> SNMYGFGTAATGEGSGVLFGNPHWYWKGPDRFYQAQLTIDGEANVSGVSFL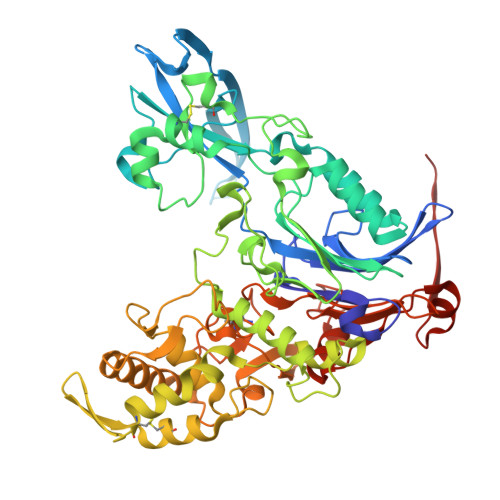GLPVIQIGFNDSVAWSHTVSTARRFGFFQLSLVQGEPTSYLRDGVPVKMKPATITVPSRNADGSVSDVTRTLYHSEFGPLVNLAGLNPALAWSQGTAFAIRDINGENFRTLRTWMRWNQAKSLDEFIAIQKEEASIPWVNTVAVGRGSAKAWYADIGAVPNVSPAQTAACTTPFGMAVGQALPNVPFFDGSRSECDWLTDADSVQKGAVGVSRMPSLQRDDYVGNMNDSYWLANVHAPLTGYPAIFGPAGTSAQTLRTRMGHTMALERLAGTDGYAGNKATSAVVREMVLGSRVFSAERFKDEVLDLICTPAQWTVNGAAVDAAQACAVLAAWDNRGRKDSRGSHLWDEFWSRVPTASLFTVPFSAADPLNTPRGINAAAADALRQAMATAIARVGQSGYALDAPRGEVLYATRGGTRLPLYGGCGAMGYFTITCSENDITQGGYSMDGQPNASNSYMQVVSFPASGVQAHTFLTFSLSDDPASPHHGDYTKAYSAGQWLRVPFTEAEITGNADYRTATVKELEHHHHHH>SSPGKPPRLVGGPMDASVEEEGVRRALDFAVGEYNKASNDMYHSRALQVVRARKQIVAGVNYFLDVEVGRTTCTKTQPNLDNC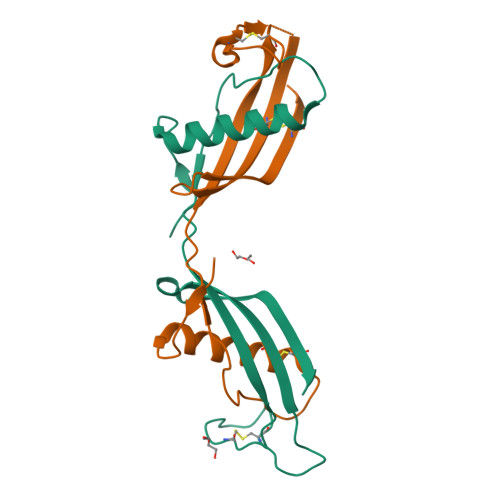PFHDQPHLKRKAFCSFQIYAVPWQGTMTLSKSTCQDA[4x]2-[3-[2,6-bis(fluoranyl)-4-(1~{H}-pyrazol-4-yl)phenyl]-3-oxidanylidene-propyl]-4-(1-methylpyrazol-4-yl)benzoic acid | C23 H18 F2 N4 O3 | 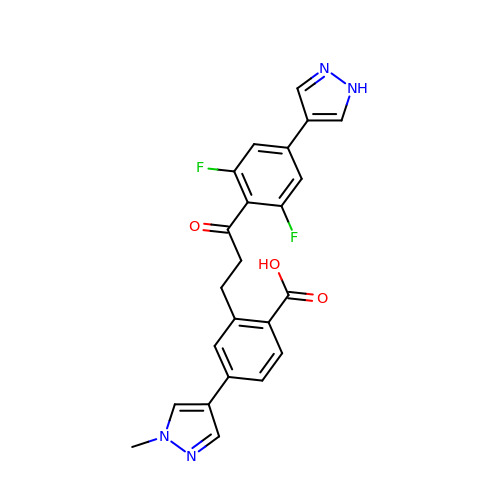NNCTWMTXMLKLDE-UHFFFAOYSA-N> SMESVADIQQLEEKVDESDVRIYFNE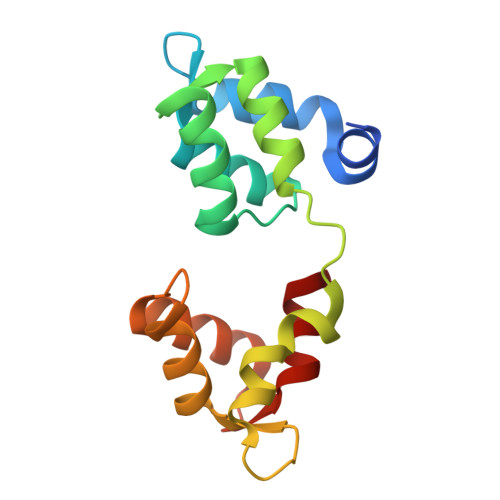KSSGGKISIDNASYNARKLGLAPSSIDEKKIKELYGDNLTYEQYLEYLSICVHDKDNVEELIKMFAHFDNNCTGYLTKSQMKNILTTWGDALTDQEAIDALNAFSSEDNIDYKLFCEDILQ[(2~{S},3~{S},4~{R},5~{R})-5-(4-azanyl-2-oxidanylidene-pyrimidin-1-yl)-2-(hydroxymethyl)-3,4-bis(oxidanyl)thiolan-2-yl] phosphono 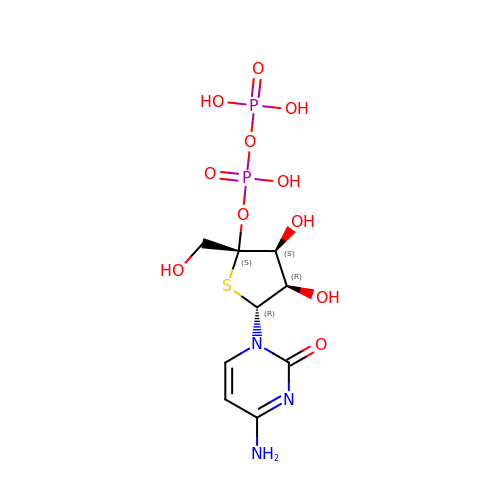hydrogen phosphate | C9 H15 N3 O11 P2 S | KEAXZHZTGMHPPH-AYHNYZOXSA-N> EGPAKKVLTLEGDLVLGGLFPVHQKGGPAEDCGPVNEHRGIQRLEAMLFALDRINRDPHLLPGVRLGAHILDSCSKDTHALEQALDFVRASLSRGADGSRHICPDGSYATHGDAPTAITGVIGGSYSDVSIQVANLLRLFQIPQISYASTSAKLSDKSRYDYFARTVPPDFFQAKAMAEILRFFNWTYVSTVASEGDYGETGIEAFELEARARNICVATSEKVGRAMSRAAFEGVVRALLQKPSARVAVLFTRSEDARELLAASQRLNASFTWVASDGWGALESVVAGSEGAAEGAITIELASYPISDFASYFQSLDPWNNSRNPWFREFWEQRFRCSFRQRDCAAHSLRAVPFEQESKIMFVVNAVYAMAHALHNMHRALCPNTTRLCDAMRPVNGRRLYKDFVLNVKFDAPFRPADTHNEVRFDRFGDGIGRYNIFTYLRAGSGRYRYQKVGYWAEGLTLDTSLIPWASPSAGPLPASRCSEPCLQNEVKSVQPGEVCCWLCIPCQPYEYRLDEFTCADCGLGYWPNASLTGCFELPQEYIRWGDAWAVGPVTIACLGALATLFVLGVFVRHNATPVVKASGRELCYILLGGVFLCYCMTFIFIAKPSTAVCTLRRLGLGTAFSVCYSALLTKTNRIARIFGGAREGAQRPRFISPASQVAICLALISGQLLIVVAWLVVEAPGTGKETAPERREVVTLRCNHRDASMLGSLAYNVLLIALCTLYAFKTRKCPENFNEAKFIGFTMYTTCIIWLAFLPIFYVTSSDYRVQTTT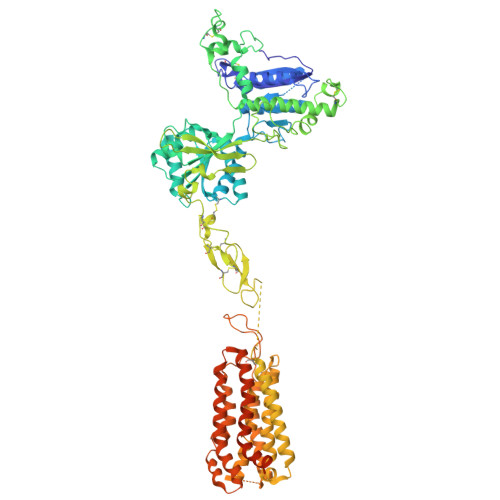MCVSVSLSGSVVLGCLFAPKLHIILFQPQKNVVSHRAPTSRFGSAAARASSSLGQGSGSQFVPTVCNGREVVDSTTSSL> RSDAAKRLL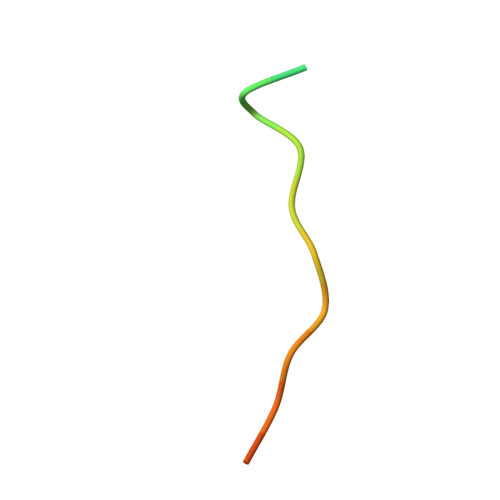EASADANIQDN>MAGSYNYAEALQKAIYFYECQQAGPLPEWNRVEWRGDATMNDEVLGGWYDAGDHVKFNLPMAYSAAMLG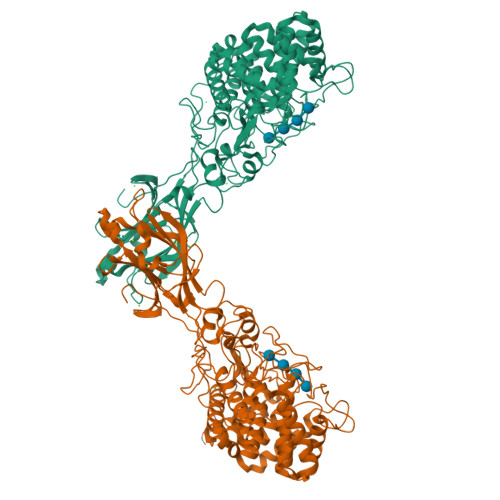WALYEYGDDIEASGQRLHLERNLAFALDYLVACDRGDSVVYQIGDGAADHKWWGSAEVIEKEMTRPYFVGKGSAVVGQMAAALAVGSIVLKNDTYLRYAKKYFELADATRSDSTYTAANGFYSSHSGFWDELLWASTWLYLATGDRNYLDKAESYTPKLNRQNQTTDIEYQWAHCWDDCHYGAMILLARATGKEEYHKFAQMHLDWWTPQGYNGKRVAYTPGGLAHLDTWGPLRYATTEAFLAFVYADSINDPALKQKYYNFAKSQIDYALGSNPDNRSYVVGFGNNPPQRPHHRTAHGTWLDKRDIPEKHRHVLYGALVGGPGRDDSYEDNIEDYVKNAVACDYNAGFVGALCRLTAEYGGTPLANFPPPEQRDDEFFVEAAINQASDHFTEIKALLNNRSSWPARLIKDLSYNYYMDLTEVFEAGYSVDDIKVTIGYCESGMDVEISPITHLYDNIYYIKISYIDGTNICPIGQEQYAAELQFRIAAPQGTKFWDPTNDFSYQGLTRELAKTKYMPVFDGATKIFGEVPGGLEHHHHHH[2x]Carotenoid cleavage oxygenases are an ancient family of enzymes that catalyze the oxidative scission of alkene substrates. The oxidative cleavage of alkene bonds by CCOs is accomplished through the use of a mononuclear non-heme iron center. It consists of an absolutely conserved set of four His residues that are arranged in a pseudo-octahedral geometry, three of which are engaged in hydrogen bonds with outer sphere Glu residues that are also highly conserved within the family. Taken together with the preceding structural data on ACO, cobalt substitution appears to preserve active site structure in CCOs without supporting catalytic activity.

The second advance was the generation of a cobalt-substituted stilbene-cleaving CCO from Neurospora crassa (CAO1) that was shown to be catalytically inert and allowed the crystallographic observation of well-resolved enzyme–substrate complexes. We previously showed that Co substitution in the stilbene-cleaving CAO1 results in undetectable catalytic activity as we have observed here for ACO. Although the previously reported crystal structure of Co-CAO1 did not show notable structural differences compared to that of Fe-CAO1, the resolution and data quality of the former structure was substantially inferior compared to the latter. To allow a more rigorous comparison, we collected data on a Co-CAO1 to a higher than previously achieved resolution, with significantly improved quality indicators. Similar to ACO, we found only minor structural differences in active site residues between Co-CAO1 and Fe-CAO1. Notably, in each monomer of the asymmetric unit, cobalt was consistently bound deeper within the 4-His metal binding pocket, in closer proximity to His197 by ~ 0.4 Å relative to iron. Additionally, we observed subtle variability in the positioning of the coordinated solvent between the two metal-bound forms of the enzyme. Like in ACO, we observed a shortening of the metal–His bond lengths in cobalt-substituted CAO1 relative to the native iron form, although the bond lengths for Fe-CAO1 could be artificially elongated owing to submaximal iron occupancy. By contrast, the cobalt ions in Co-CAO1 have B-factors that are comparable to the coordinating His Nε atoms indicating full cobalt occupancy at the metal-binding site. Our pre-edge analysis, therefore, supports a five-coordinate geometry for the cobalt site in both CAO1 and ACO.

>MAEYVFSDAPKDSHGNGVKDAVPGKQPEELPPAPRYFQGENTAGFMRPVRFEGDITNLEVVGEIPKSIEGTFYRVMPEPHLPSFIPNDPWFNGDGNISGFYFKDGHVDLKQRYVRTEKFVREAEARRSLLGKYRNRYTDLVEFKIRSTANTNIVYWRGQLLALKEDSPPYAMDPETLETFGVYDFDGQLPSLTFTAHPKFDPVTREMVCFGYEAKGDGTRDICYYSFGPDGKIAETVWLVSPVCGMIHDFAVTENFVIFPIIPLVCDVERMKQGGDHWQWDYSIPMYIGVLPRRGAQGSDVKWFEAPHGFAGHVANAFEDDKGHIQLQMAYAKDNVFFWWPDANGKGPRPGEVEAHFANFVLDYQSDKLPLAEPTYLVDDDMEFPRIDDRVATRKHKHTFFCIFDRKPGVTDFEFVMPRAGGGAPMSNGLAHLNHETGDIQRYLPGPRKLTGECIFIPRNSEAAEGDGYVMVLLANYEDMCSELAVLDTKDLTNEVALIKLPVRLRPGLHGNWVDKSDVDGHPAPL[4x]> MSVLDALWEDRDVRFDVSSQQMKTRPGEVLIDCLDSVEDTKGNNGDRGRLLVTNLRIVWHSLALPRVNLSIGYNCILNITTRTANSKLRGQTEALYVLTKCNSTRFEFIFTNLVPGSPRLYTSLIAVHRAYETSKMYRDFKLR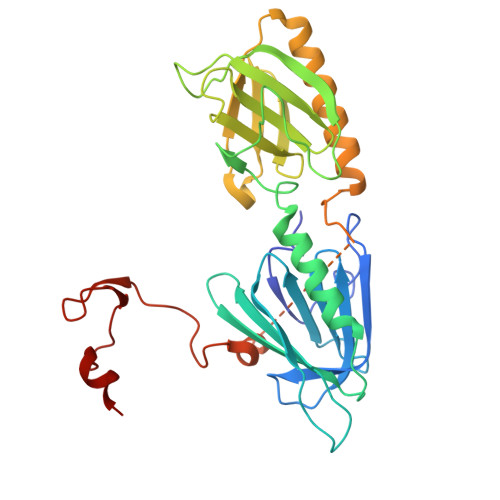SALIQNKQLRLLPQENVYNKINGVWNLSSDQGNLGTFFITNVRIVWHANMNDSFNVSIPYLQIRSVKIRDSKFGLALVIESSQQSGGYVLGFKIDPVEKLQESVKEINSLHKVYSANPIFGVDYEMEEKPQPLEALTVKQIQDDVEIDSDDHTDAFVAYFADGNKQQDREPVFSEELGLAIEKLKDGFTLQGLWEVMN> GFGCNGPWDEDDMQCHN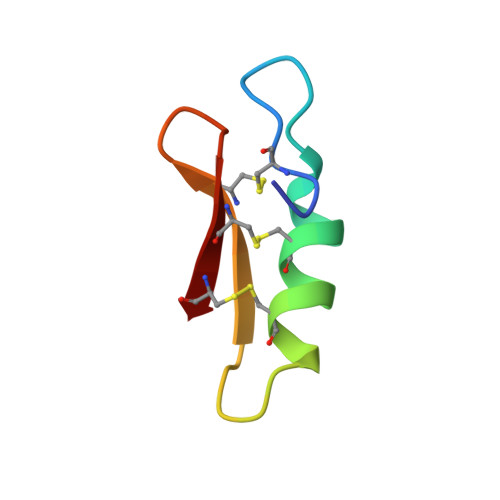HCKSIKGYKGGYCAKGGFVCKCY> S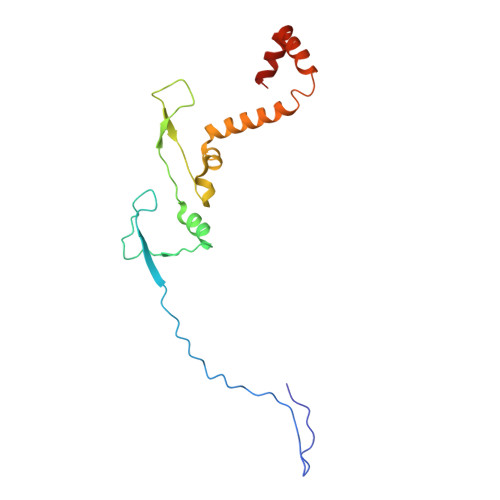KEGSVAPKERINIKYIPATGDAQAEVAEVELPLKTLVVGDFKGHAEQTPLEERATVTVDKNNFEAVMRESELKITATVKNKLTDDENAELPVELNFKSLADFAPDAVASQVPELKKLIELREALVALKGPLGNIPAFRERLQSLLNSEESREKLLAEL> GSAKDPSLPERIDTFTELFNYEVALKSYDIRILQSNYPTKLLSPDSLLPQTSDYPLKDIQQLYSLANTCRGKLPLSPLITEPLVFTRAICKGTQLT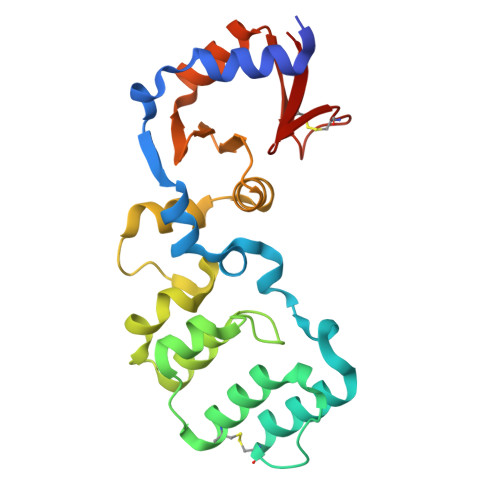PRWFSRSGLIHPGGGTYAARYVEKYPELRPKLAQYMHIKERDNEEGDELLESLQNMDDDAINALIAGASMFIEGKEMWLRRGDRYFVFSKDVWQENVANAGLSYTLASQSKSCFVKRGNICWDVE>[16x]MKIAVLSRNPRLYSTRRLVEAGIERGHEMVVIDTLRAYMNIASHKPQIHYRGKPLEGFDAVIPRIGASVTFYGCAVL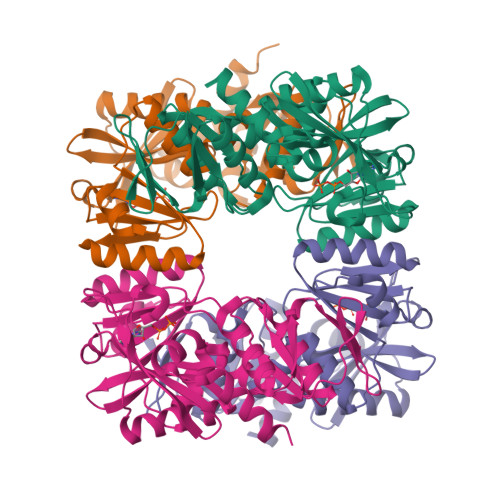RQFEMMGVFPLNESVAIARSRDKLRSLQLLSRRGIGLPVTGFAHSPDDIPDLIQMVNGAPLVIKVLEGTQGIGVVLCETATAAESVIEAFMGLKQDIMVQEYIKEAGGADIRCFVVGDKVIASMKRQAKPGEFRSNLHRGGSASLIKITPEERMTALRAAKVMGLSVAGVDILRSNHGPLVMEVNSSPGLEGIEVTTSKDVAGMIIEYLEKNSGPHMTRTKGKGLEHHHHHH>[6x]NAMALAAPPGELTLALTPDDKTLDPASLDRALAILAEHGILVLTGMLRTRLTDQLRTAMLDDLPEVLRQQDVPTNFVPGHVQQDPPVRESLLFPDVLL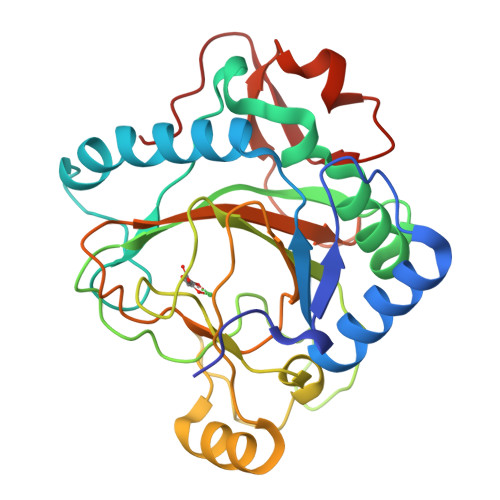NPVVYQITHAVLGADARNAVYSGNMNLPGSHEQPVHLDEPHLWPGISHPPYCLCVDVPLIDFTLENGSTEYWPGSHVLNPDECYDERGCVLPAELERRRAVAPPVRFPIPVGSVVIRDGRLWHRGVPNLSAAPRPLLAMTHYTEWFDMPPIQLPDTVKSWVDGSDRHTHAHFVAGDVDHLT tert-butyl [(1R,3R)-3-(imidazo[4,5-d]pyrrolo[2,3-b]pyridin-1(6H)-yl)cyclopentyl]carbamate | C18 H23 N5 O2 | 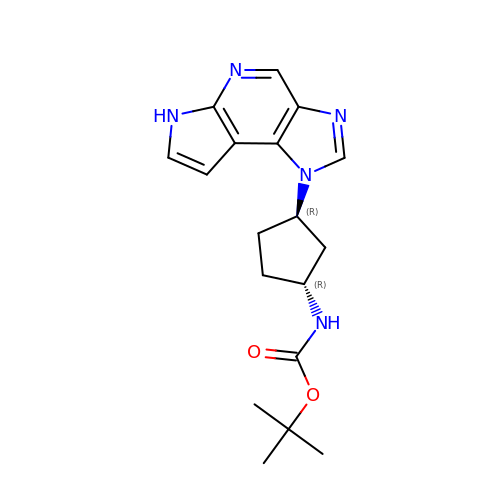GAVWHEZXKOVIQY-VXGBXAGGSA-N> MVAGAVAGALIGAAVVAATAATGGLAAVILAGSIAAGGLSMFQIVKGLTTIFELPEPTTGVLIRGSFNVYVNSRNAMRAGDDVSATCSGLPLNHPLWPFPVLIAEGSATVYINGKPAARLQSKMVCGAHIKTGSQ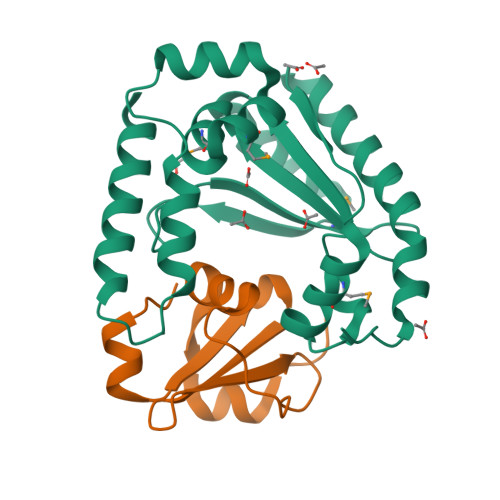NTFIGGPTERVAFVLDLEEWLHTGLEALGLAALAGGLLLAAMAGVAALVGVVAIGGLMMGGMALLGDLGDRLGPGYRDLFQGVAGMALLGFGPKMARLGNAPKGAPKTQVPKGFEKVYGKAPAAKAEIDAVADGLAAKHGGRVAKAPIKSRERAMQKINNDYKGDPTKIKDLARNTIIVEGDKVNTVAAELANRGAKVKVIDGNADPLGYSGVNSTMNTKAGIPGEIQVNSPEMIYAKESEDMARILLGNDTYDAVAAKAGVPGGQGHKYYEDWRVLDPKSPEAQAIAEKSRAYYDAVRKGNGN;> MAIEKGEAFARRDIYIDYDFEDVTYRWDHRQGTIHVRFYGEAESPEPVEHDNRLFNDALRFGREITREEYETGFPKG>MNPNQKIITIGSVCMTIGMANLILQIGNIISIWISHSIQLGNQNQIETCNQSVITYENNTWVNQTYVNISNTNFAAGQSVVSVKLAGNSSLCPVSGWAIYSKDNSIRIGSKGDVFVIREPFISCSPLECRTFFLTQGALLNDKHSNGTIKDRSPYRTLMSCPIGEVPSPYNSRFESVAWSASACHDGINWLTIGISGPDNGAVAVLKYNGIITDTIKSWRNNRLRTQESECACVNGSCFTVMTDGPSDGQASYKIFRIEKGKIVKSVEMNAPNYHYEECSCYPDSSEITCVCRDNWHGSNRPWVSFNQNLEYQIGYICSGIFGDNPRPNDKTGSCGPVSSNGANGVKGFSFKYGNGVWIGRTKSISSRNGFEMIWDPNGWTGTDNDFSIKQDIVGINEWSGYSGSFVQHPELTGLDCIRPCFWVELIRGRPK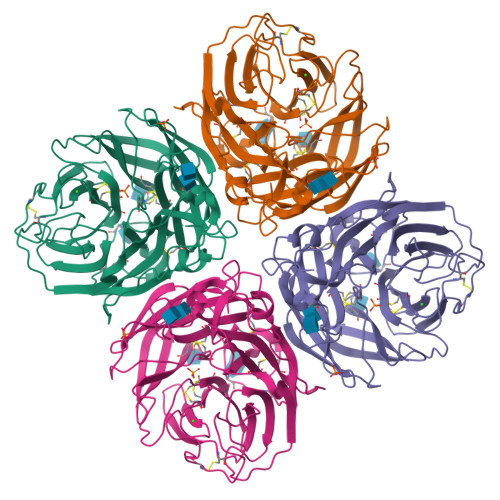ENTIWTSGSSISFCGVNSDTVGWSWPDGAELPFTIDK[2x]> SRWMEPYFDPSTPRNVTALMGKSAYLSCRVRNLANKTVSWIRHRDIHILTVGSYTYTSDQRFQATHHQDTEDWTLQIKWAQKRDAGMYECQISTQPVRSYFV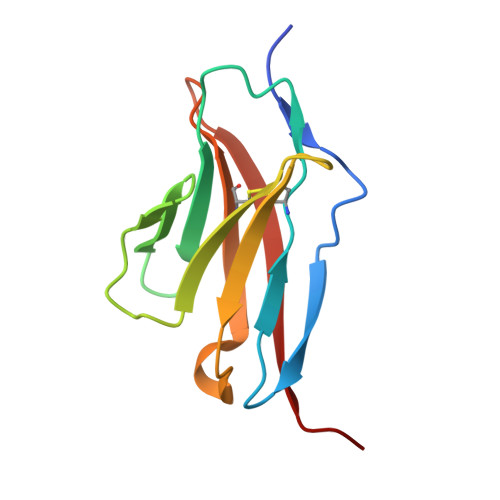RLNVVVPH>[2x]SMGLVETLRRFRGDVTLDPDTANPELILSEDRRSVQRGDLRQALPDSPERFDPGPCVLGQERFTSGRHYWEVEVGDRTSWALGVCRENVNRKEKGELSAGNGFWILVFLGSY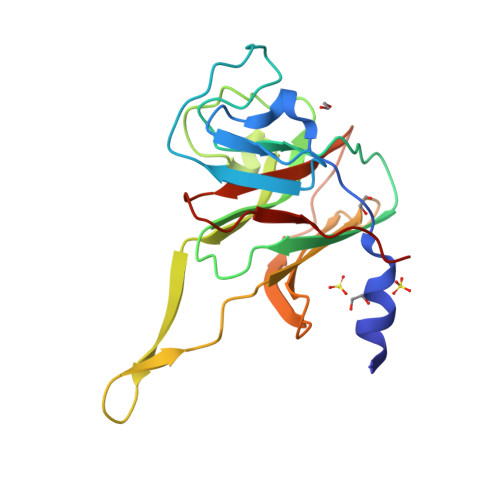YNSSERALAPLRDPPRRVGIFLDYEAGHLSFYSATDGSLLFIFPEIPFSGTLRPLFSPLSSSPTPMTICRPKGGS4-[(8-{4-[(E)-2-cyanoethenyl]-2,6-dimethylphenyl}-6-oxo-5,6,7,8-tetrahydropteridin-2-yl)amino]benzonitrile 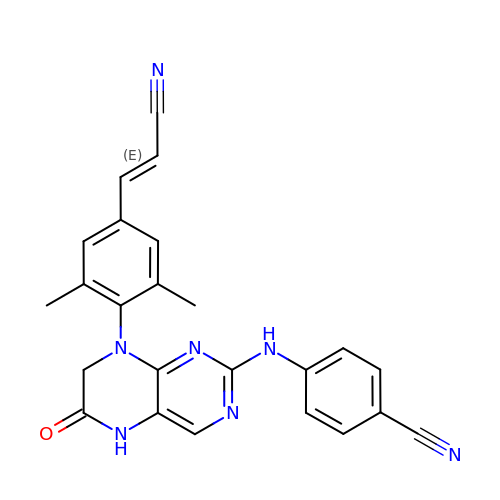| C24 H19 N7 O | QRFWWEONRMHITJ-ONEGZZNKSA-N> MDDKELIEYFKSQMKEDPDMASAVAAIRT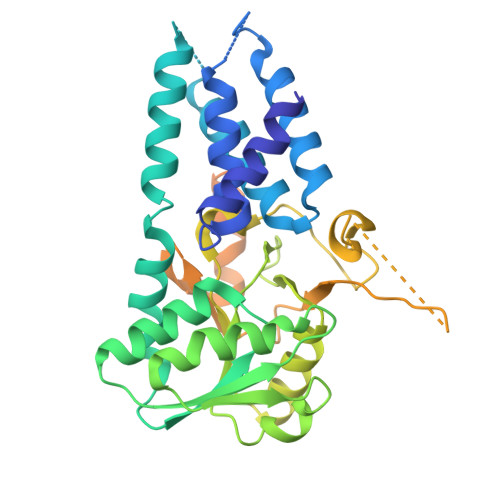LLEFLKRDKGETIQGLRANLTSAIETLCGVDSSVAVSSGGELFLRFISLASLEYSDYSKCKKIMIERGELFLRRISLSRNKIADLCHTFIKDGATILTHAYSRVVLRVLEAAVAAKKRFSVYVTESQPDLSGKKMAKALCHLNVPVTVVLDAAVGYIMEKADLVIVGAEGVVENGGIINKIGTNQMAVCAKAQNKPFYVVAESFKFVRLFPLNQQDVPDKFKYKADTLKVAQTGQDLKEEHPWVDYTAPSLITLLFTDLGVLTPSAVSDELIKLYLGGENLYFQAEDKGGGSGGGGSGGGGSASQGGLNDIFEAQKIEWHEGGGGSGGGGSGGGGSGRDQDYKDDDDK> GAQVSTQKTGAHETSLSASGNSIIHYTN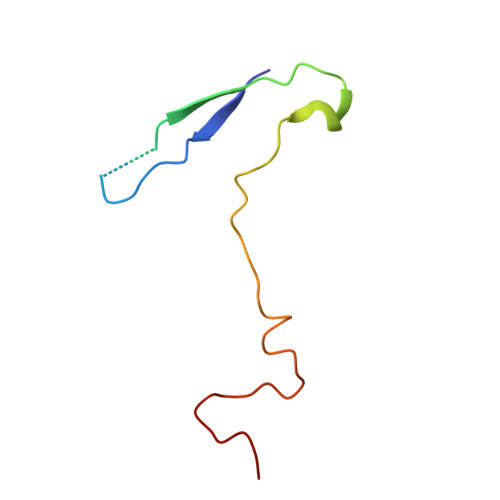INYYKDAASNSANRQDFTQDPGKFTEPVKDIMVKSLPALN> MKV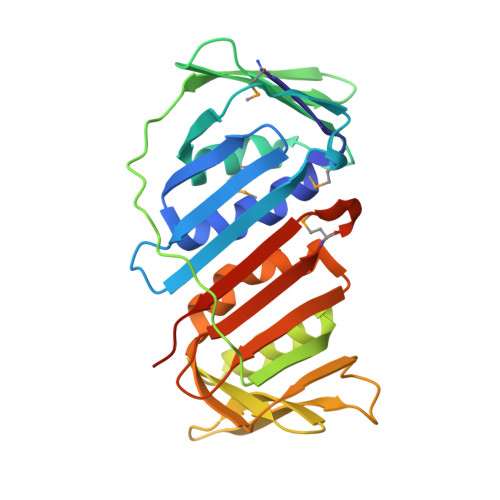VYDDVRVLKDIIQALARLVDEAVLKFKQDSVELVALDRAHISLISVNLPREMFKEYDVNDEFKFGFNTQYLMKILKVAKRKEAIEIASESPDSVIINIIGSTNREFNVRNLEVSEQEIPEINLQFDISATISSDGFKSAISEVSTVTDNVVVEGHEDRILIKAEGESEVEVEFSKDTGGLQDLEFSKESKNSYSAEYLDDVLSLTKLSDYVKISFGNQKPLQLFFNMEGGGKVTYLLAPKVLEHHHHHH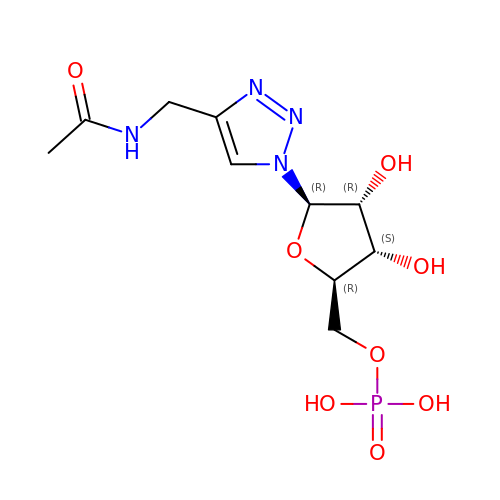[(2~{R},3~{S},4~{R},5~{R})-5-[4-(acetamidomethyl)-1,2,3-triazol-1-yl]-3,4-bis(oxidanyl)oxolan-2-yl]methyl dihydrogen phosphate | C10 H17 N4 O8 P | WKSDLIPBAPRDGN-ZYUZMQFOSA-N>MGVPIGDLVPRKEIDLENLYGKKIAIDALNAIYQFLSTIRQEDGTPLMDSKGRITSHLSGLFYRTINLMEAGIKPAYVFDGKPPEFKRKELEKRREAREEAELKWKEALAKGNLEEARKYAQRATKVNEMLIEDAKKLLQLMGIPIIQAPSEGEAQAAYMASKGDVYASASQDYDSLLFGAPRLIRNLTITGKRKMPGKDVYVEIKPELVVLDEVLKELKITREKLIELAILVGTDYN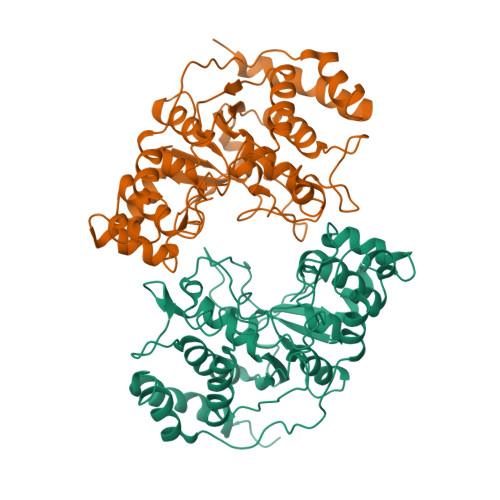PGGVKGIGPKKALEIVRYSRDPLAKFQRQSDVDLYAIKEFFLNPPVTNEYSLSWKEPDEEGILKFLCDEHNFSEERVKNGIERLKKAIKAGRQSTLESWFVKKKP[2x]> MSTSSHTVLLIQTSPRLDSRTWGDYESVTDALDALCKMFEDFLSKKSAAPVTYDVSQVYEFLDKLSDVSMMIFNRETGQYIGRTRAWIKQQVYEMMRGRCQHPGSSGSSGSSGSSGSSGSSGSSNKRITLNERFGVLEKGYTIQA;> MSTSSHTVLLIQTSPRLDSRTWGDYESVTDALDALCKMFEDFLSKKSAAPVTYDVSQV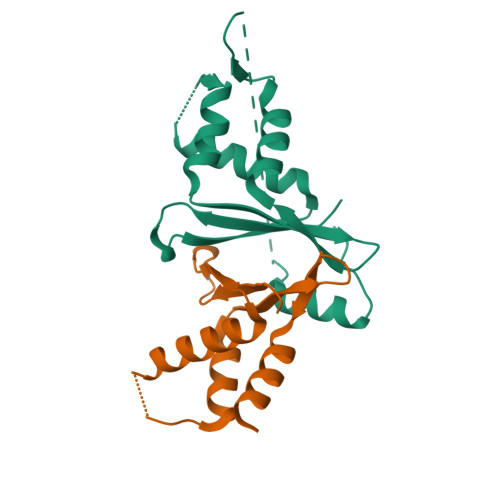YEFLDKLSDVSMMIFNRETGQYIGRTRAWIKQQVYEMMRGRCQHPG> GAASEIEKRQEENRKDREKAAAKFREYFPNFVGEPKSKDILKLRLYEQQHGKCLYSGKEINLGRLNEKGYVEIDHALPFSRTWDDSFN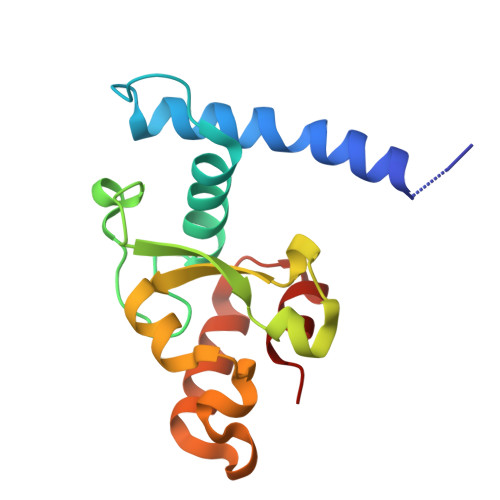NKVLVLGSENQNKGNQTPYEYFNGKDNSREWQEFKARVETSRFPRSKKQRILLQ In this study, we take advantage of a recently identified prokaryote homologue of HCN and CNG channels, termed SthK, which originates from the thermophylic bacterium Spirochaeta thermophila. We previously demonstrated that SthK is gated by cAMP, but not cGMP, and is relatively insensitive to voltage, which resembles the gating properties of certain eukaryote CNG channels. Using X-ray crystallography, we determined the 3-dimensional structures of the isolated C-linker/CNBD of SthK, termed SthK-Cterm, in complex with cAMP or cGMP. The C-linker domain is followed by the CNBD, which contains four helices (αA, αB, αP, αC) and eight β-strands arranged in a so-called β-roll, which is flanked by the A- and B-helices.

The crystal structure of SthK-Cterm in complex with cGMP, which is an antagonist, adopts an overall architectural fold that strongly resembles that of previous structures of HCN C-terminal domains. Additionally, the structure of SthK-Cterm in complex with cGMP, which is an antagonist, shows the SthK-Cterm in a more closed conformation which is similar to the conformations which were previously shown for HCN2 C-terminal structures. In the structure of cGMP-bound SthK-Cterm we observe that cGMP is able to bind in the cyclic nucleotide binding cavity from SthK. Moreover, the phosphoribose group from cGMP establishes the same interactions that were described earlier for the phosphoribose group from cAMP in the SthK-Cterm structure. Remarkably, we observe that cGMP is bound in its anti-conformation in SthK-Cterm whereas previously published cGMP-bound CNBD structures showed the cGMP molecule bound in its syn conformation. The anti-conformation in the cGMP-bound SthK-Cterm structure prevents the purine ring of cGMP from establishing binding interactions with the C-helix or Thr-378 from the CNBD. Therefore, it is possible that antagonism by cGMP arises from missing interactions between the purine ring of cGMP and the C-helix of SthK. Moreover, the SthK-Cterm crystal structure suggests that binding of the cGMP molecule in the syn conformation might be prevented by the presence of the Leu-422 residue which enters the cGMP binding pocket and is equivalent to the Asp residue which has been described to play an important role in cGMP specificity. Therefore, this differential orientation might explain why cGMP acts as an agonist in HCN2 channels but as an antagonist in the SthK channel. Most likely, the absence of these interactions explains why binding of cGMP to SthK does not provide the required energy for the opening conformational changes.

>DAAKLLHRERMERVTAFLSYKKISPELQRRILEYFDYLWETRRGYEEREVLKELPHPLRLAVAMEIHGDVIEKVPLFKGAGEDFIRDIILHLEPVIYGPGEYIIRAGELGSDVYFINRGSVEVLSADEKTRYAILSEGQFFGEMALILRAPRTATVRARTFCDLYRLDKETFDRILSRYPEIAAQIQELAVRRKEELE[2x]> MSAIKPDMKIKLRMEGNVNGHHFVIDGDGTGKPFEGKQSMDLEVKEGGPLPFAFDILTTAFLYGNRVFAKYPDNIQDYFKQSFPKGYSWERSLTFEDGGICIARNDITMEGDTFYNKVRFYGTNFPANGPVMQKKTLKWEPSTEKMYVRDGVLTGDVEMALLLEGNAHYRCDFRTTYKAKEKGVKLPGAHFVDHCIEILSHDKDYNKVKLYEHAVAHSGLPDNARR

The mGeos series of rsFP’s display similar switching behavior to Dronpa. The series was developed from mEos2, with mutations that remove the undesirable irreversible green-to-red photo conversation, increase fluorescence brightness and provide high thermal stability of the off-state. Skylan-NS represents a further improvement, with reduced per cycle bleaching and higher photoswitching quantum yield in the on→off than Dronpa. We present high resolution room temperature SFX structures of Skylan-NS in both ‘on’ and meta-stable ‘off’ state collected using two different XFELs, the SPring-8 Angstrom Compact free electron Laser (SACLA), Japan and the Linear Coherent Light Source (LCLS), USA.

The higher resolution datasets, both collected for the off-state after saturating green illumination and were readily phased by molecular replacement with 10.02 and 9.27 sigma solutions. The two off-state datasets go to higher resolution, but mainly due to the higher photon energy and short detector distances used during these beam times. A remarkable agreement was found between the LCLS and SACLA datasets of the off-state for resolution below 2 Å, while the R-factor is also reasonable for the higher resolution terms (Red). The R-factor for the on- and off-state experiments using the droplet methods (green) (but at different photon energy) is considerably higher than the two off-state measurements conducted at different facilities, including the lower resolution reflections. Similarly, both off-state structures were seen to have trans chromophore conformations with full occupancy, giving no indication for the presence of on-state with cis conformation in conventional and omit difference maps. Considering that optical measurements also showed negligible bleaching with full conversion, the off-state crystal structures are found to represent the pure photoisomerisation product and not a mixture of photo products. Photoisomerisation is clearly seen in a comparison of the “on” and “off” refined structures where the dihedral angle of the chain connecting the phenol ring to the rest of the chromophore (N–C=C–C) changes from 1° (cis) → 171.1° (trans) in the on- vs the off-state and the pheonolic oxygen is displaced by 6.2 Å. In this off-state the chromophore phenol ring has been repositioned to include an indirect hydrogen bonding via an ordered water to the carboxylate of glutamate-144. In the off-state of Skylan-NS, the hydrogen bonding distances are 2.4 Å and 2.6 Å between the phenolic oxygen and water, and water and carboxylate respectively. The Arg-66 side chain also displays a translation/extension motion where the direct hydrogen bonding between the guanidinium group and the oxygen of the chromophores’ imidazolic base can been disrupted and Arg-66 has been pulled “below” the chromophore by it binding to Glu-144 and the newly displaced His-194, resulting in a total movement of 2.6 Å towards His-194.>MDLEYMHISYPNILLNMRDGSKLRGYFAKKYIDEEIVHNHRDNAFVYKYPQIQFKIIDRSPLIIGIGSLGINFLESKRIFFEKELIISNDTNDITEVNVHKDMDHFGTTDKILKYQFKTPWMALNAK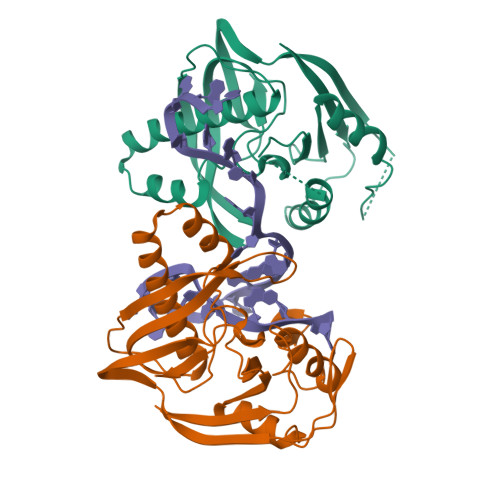NSEIYKNSDEIDREEFLKRVLIGNILSMSKSLGYTIEEKLKVKINLKEVPVKFKNQNMVGFRGEFYINFDIPQYLGIGRNVSRGFGTVVKV[2x]> FP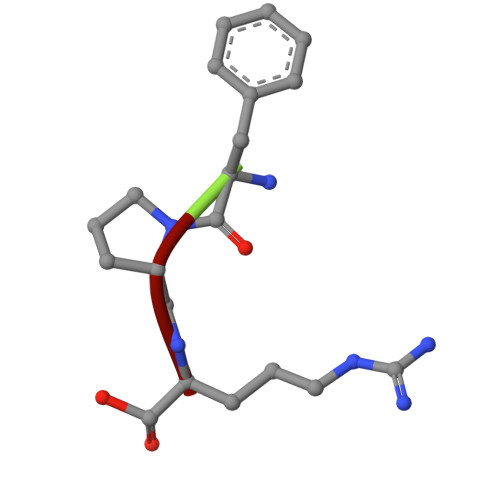R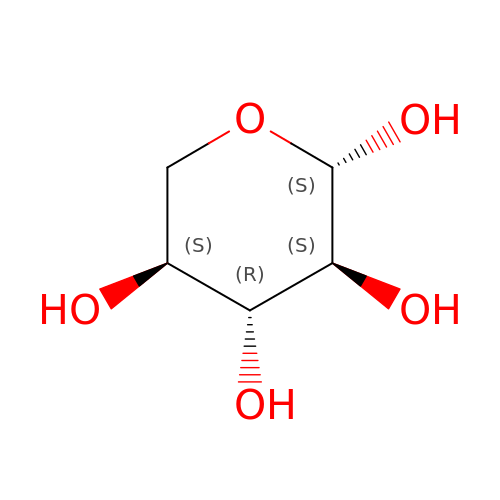beta-L-xylopyranose | C5 H10 O5 | SRBFZHDQGSBBOR-QTBDOELSSA-N> MIEIESLSRKWKNFSLDNLSLKVESGEYFVILGPTGAGKTLFLELIAGFHVPDSGRILLDGKDVTDLSPEKHDIAFVYQNYSLFPHMNVKKNLEFGMRMKKIKDPKRVLDTARDLKIEHLLDRNPLTLSGGEQQRVALARALVTNPKILLLDEPLSALDPRTQENAREMLSVLHKKNKLTVLHITHDQTEARIMADRIAVVMDGKLIQVGKPEEIFEKPVEGRVASFVGFENVLKGRVISAEQGLLRIRVGEVVIDAAGDM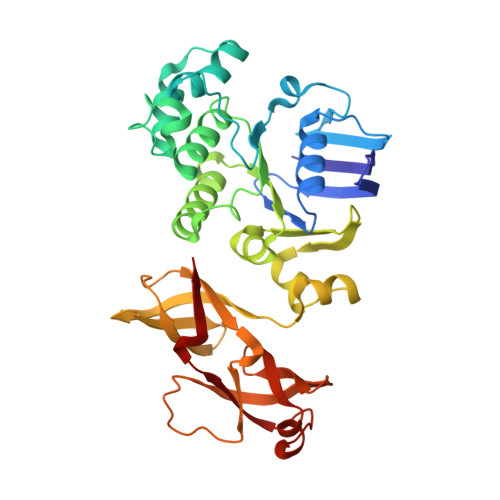EVGDQVYAFLRPENIALSKSSTQSSIRNSLQGRVTEAWVLGALVRVKVDCGVPLNVLITRRSAEEMELSPGVQIYARFKASSVHVLR> ANSLVEEFKSGNIERECIEERCSKEEAREVFEDDE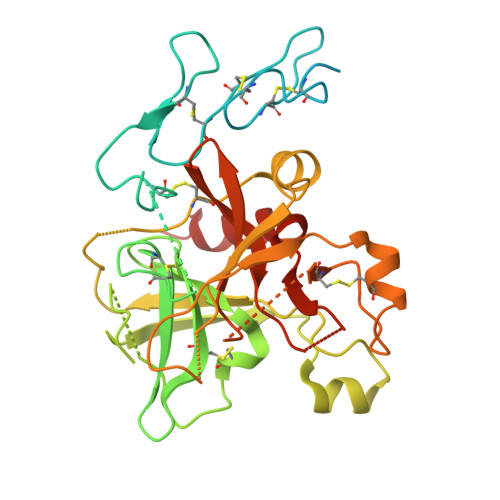KTETFWNVYVDGDQCSSNPCHYRGICKDGIGSYTCTCLSGYEGKNCERVLYKSCRVDNGNCWHFCKHVQNDIQCSCAEGYLLGEDGHSCVAGGNFSCGRNIKTRNKREANLPDFVQSQNATLLKKSDNPSPDIRIVNGMDCKLGECPWQAALVDEKEGVFCGGTILSPIYVLTAAHCINETETISVVVGEIDKSRIETGPLLSVDKIYVHKKFVPPQKAYKFDLAAYDYDIAIIQMKTPIQFSENVVPACLPTADFANQVLMKQDFGIVSGFGRIVEKGPKSKTLKVLKVPYVDRHTCMVSSETPITPNMFCAGYDTLPRDACQGDSGGPHTTVYRDTHFITGIVSSGEGCARNGKYGNYTKLSKFIPWIKRIMRQKLPSTESSTGRL>MTTSYEPWPQLYSHLNGTNEEVLDRMKVAELCKGWSVYRDASEWANFKEMFTPDANIWTTWSGAQTIDSFIQISKDGKDKGAFIMHRECGTLVDLNPKTQRAIGKMKTTITQRFEYEGVPFDIDCDNYFIFFCLKDSNGDWKARWYKVFYVKDKFVPVG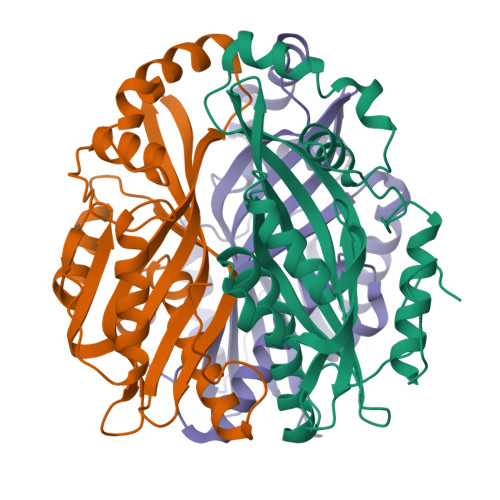VPTAENMEKLAKLFSKENLEQYPWGYQYLAVAQANLGYPIDKKLPTWKNELYHTMYDAMKEWMEGKEIDLHW[9x]N-(2-aminopyridin-3-yl)acetamide 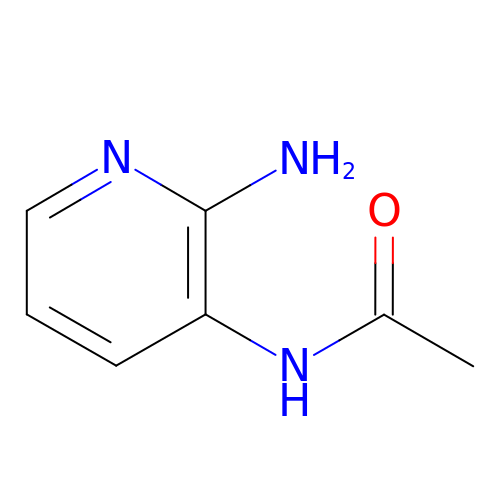| C7 H9 N3 O | HMDOCRZUNBZAGA-UHFFFAOYSA-N>[2x]SSRELIEREASIQAEMRTSMQYVDRTVGKATSIFILDDSKFKGSKQGLTREWSYIGLSADGKKVMNYVWNKQKQDWDVSELGTKSLYNMKLDLEFKTEGAYQDNRLISYNLTGKYPDTNNKLGIDTAISALNTKQVFSKVAKGKKGIAIAYRTDPIQGQMNIAVSFVFDTSGSMDWDLQGRNVKKTGNESRMDILRKKSVIMIKDLAEIGNISVNLVGFSTSAKYIQQNFSNLDNGTNTIIATI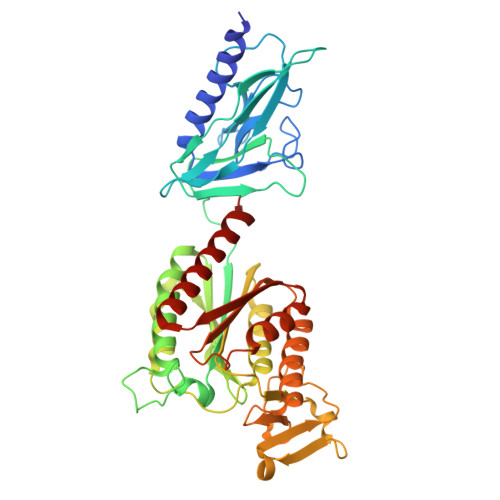TKRENLNPDGVTNPGDGLRYGMISLQSQPAQLKYIVLLTAGIPNAYLVDSRALYAGNRVDLSQGAGRVTFNNPIYDLSPTLGYEYSRLGYDLYSRDSITRENSIAYAGEVSKKFGLGIKRVNVIGFSGVNHEIAYGQSLTDRIGEGGMETKYVSATNEEALQKTFSDIKKQIQQDLWFVSGP> MSSGRIIQIIGAVIDVEFERTSVPKIYDALQVDGTETTLEVQQQLGDGVVRTIAMGSTEGLKRGLTVTSTNAPISVPVGTATLGRIMDVLGRPIDEAGPVATEERLPIHRQAPSYAEQAASTDLLETGIKVIDLLCPFAKGGKVGLFGGAGVGKTVNMMELINNIAKAHSGLSVFAGVGERTREGNDFYHEMKDSNVLDKV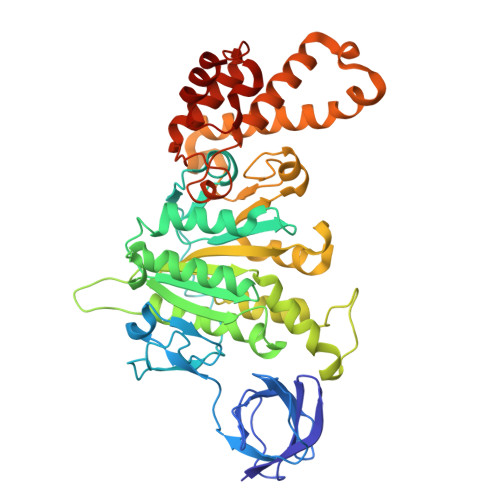AMVYGQMNEPPGNRLRVALTGLTMAEYFRDEKDENGKGRDVLLFVDNIYRYTLAGTEVSALLGRMPSAVGYQPTLAEEMGVLQERITSTKSGSITSIQAVYVPADDLTDPSPATTFAHLDATVVLSRDIASSGIYPAIDPLDSTSRQLDPLVVGQEHYEIARAVQNVLQRYKELKDIIAILGMDELAEEDKLVVYRARKIQRFFSQPFHVAEVFTGAPGKLVPLKETIRGFKGLLAGEYDHIPEQAFYMVGGIDEVIAKAEKL>TLSEKIHHPITEQGGESDLSSFAPDAASITSSIKYHAEFTPVFSPERFELPKAFFATAQSVRDSLLINWNATYDIYEKLNMKQAYYLSMEFLQGRALLNAIGNLELTGAFAEALKNLGHNLENVASQEPDAALGNGGLGRLASCFLDSLATLNYPAWGYGLRYKYGLFKQRITKDGQEEVAEDWLEIGSPWEVVRNDVSYPIKFYGKVSTGSDGKRYWIGGEDIKAVAYDVPIPGYKTRTTISLRLWSTQVPSADFDLSAFNAGEHTKACEAQANAEKICYILYPGDESEEGKILRLKQQYTLCSASLQDIISRFERRSGDRIKWEEFPEKVAVQMNDTHPTLCIPELMRILIDLKGLNWNEAWNITQRTVAYTNHTVLPEALEKWSYELMQKLLPRHVEIIEAIDEELVHEIVLKYGSMDLNKLEEKLTTMRILENFDLPSSVAELFIKPEISVDDDTETVEVHDKVEASDKVVTNDEDDTGKKTSVKIEAAAEKDIDKKTPVSPEPAVIPPKKVRMANLCVVGGHAVNGVAEIHSEIVKEEVFNDFYELWPEKFQNKTNGVTPRRWIRFCNPPLSAIITKWTGTEDWVLKTEKLAELQKFADNEDLQNEWREAKRSNKIKVVSFLKEKTGYSVVPDAMFDIQVKRIHEYKRQLLNIFGIVYRYKKMKEMTAAERKTNFVPRVCIFGGKAFATYVQAKRIVKFITDVGATINHDPEIGDLLKVVFVPDYNVSVAELLIPASDLSEHISTAGMEASGTSNMKFAMNGCIQIGTLDGANVEIREEVGEENFFLFGAQAHEIAGLRKERADGKFVPDERFEEVKEFVRSGAFGSYNYDDLIGSLEGNEGFGRADYFLVGKDFPSYIECQEKVDEAYRDQKRWTTMSILNTAGSYKFSSDRTIHEYAKDIWNIEAVEIA[3x]

Starch phosphorylase (EC 2.4.1.1, α-d-glucosyl transferase; SP) catalyzes the reversible conversion of starch and inorganic phosphate into glucose-1-phosphate (Glc-1-P), playing an important role in starch metabolism in plants. S. tuberosum phosphorylase is the first starch phosphorylase discovered3−5 and has served as a model SP for biochemical studies of plant phosphorylases. The most significant structural difference between the Pho1 and Pho2 forms is a 78-residue-long peptide insertion in the middle of Pho1, termed the L78 segment. The stPho1ΔL78 structure reveals that activation of the enzyme occurs through the proteolytic degradation of the L78 segment and the association of the two remaining protein segments to form the active enzyme.

In the crystal structure of the stPho1ΔL78-β-CD complex, one β-CD molecule was found in each one of the three molecules of stPho1ΔL78 crystallographic trimer with B factors around 170 Å2. The β-CD molecule binds at a totally different location from the glycogen storage binding site in rmGPb. The β-CD binding site (named glucan binding site thereafter) is situated on the surface of the protein molecule approximately 20 Å from the catalytic site. It is a shallow cavity composed of three loops. The stPho1 glucan binding site is at the entrance of a channel leading to the active site and β-CD is bound at the one edge of this channel encapsulating the side chain of Phe848 where the other part of β-CD packs against the side chain of Tyr853. There, the glucose residues of β-CD, G2, G3, and G4 are involved in five hydrogen bonds with the main chain atoms of Gly847, Phe848, and Gly849 and the side chain of Glu650. Furthermore, G2–G6 are involved in 55 van der Waals interactions with stPho1ΔL78 residues. The binding of β-CD seems to obstruct the entrance to the channel that leads to the active site. Hence, the strong inhibition displayed by β-CD for stPho1 could be attributed to this. In the HvPho1 structure, the binding of maltotetraose triggers a conformational change of a loop between Thr422 and Ala427 from an open to a more closed conformation, but such a conformational change is not observed in the stPho1ΔL78 structure upon binding of β-CD and the corresponding loop remains in the open conformation.> MFFDELKIDNKVDIIGNNVRGELPNIWLQYGQFKLKASGGDGTYSWYSENTSIATVDASGKVTLNGKGSVVIKATSGDKQTVSYTIKAPSYMIKVDKQAYYADA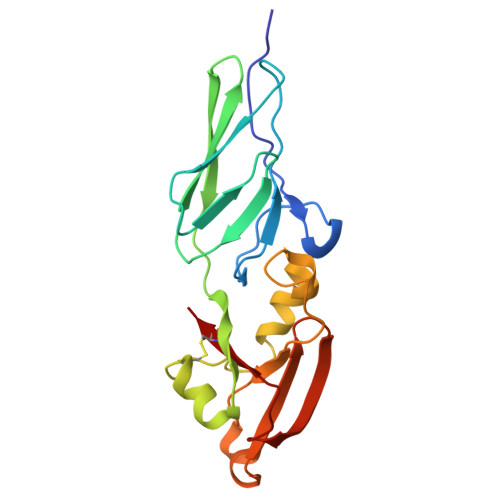MSICKNLLPSTQTVLSDIYDSWGAANKYSHYSSMNSITAWIKQTSSEQRSGVSSTYNLITQNPLPGVNVNTPNVYAVCVE>[2x]MNTDDILFSYGEEDIPLKALSFPIFETTNFYFDSFDEMSKALRNGDYEFVYKRGSNPTTRLVEKKLAALEECEDARLVASGMSAISLSILHFLSSGDHVVCVDEAYSWAKKFFNYLS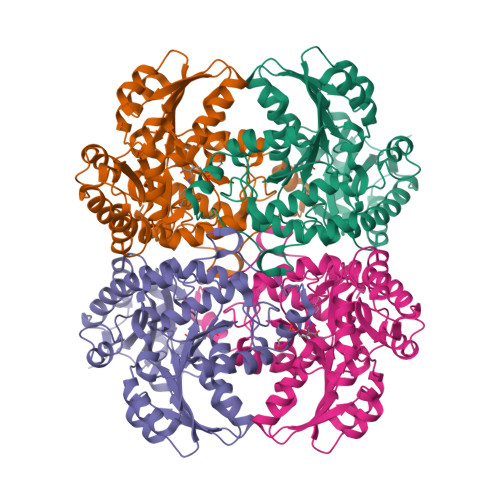KKFDIEVSYVPPDAERIVEAITKKTKLIYLESPTSMRMKVIDIRKVTEAAGELKIKTVIDNTWASPIFQKPKLLGVDVVVHSATKYISGHGDVMAGVIAGDVEDMKNIFVDEYKNIGPVLSPIEAWLILRGLRTLELRMKKHYENALVVSDFLMDHPKVLEVNYPMNPRSPQYELASSQMSGGSGLMSFRLKTDSAEKVKEFVESLRVFRMAVSWGSHENLVVPRVAYGDCPKKDVNLIRIHVGLGDPEKLVEDLDQALKKIAAALEHHHHHHHH> MRVDELRVDERIKSTLKERGIESFYPPQAEALKSGILEGKNALISIPTASGKTLIAEIAMVHRILTQGGKAVYIVPLKALAEEKFQEFQDWEKIGLRVAMATGDYDSKDEWLGKYDIIIATAEKFDSLLRHGSSWIKDVKILVADEIHLIGSRDRGATLEVILAHMLGKAQIIGLSATIGNPEELAEWLNAELIVSDWRPVKLRRGVFYQGFVTWEDGSIDRFSSWEELVYDAIRKKKGALIFVNMRRKAERVALELSKKVKSLLTKPEIRALNELADSLEENPTNEKLAKAIRGGVAFHHAGLGRDERVLVEENFRKGIIKAVVATPTLSAGINTPAFRVIIRDIWRYSDFGMERIPIIEVHQMLGRAGRPKYDEVGEGIIVSTSDDPREVMNHYIFGKPEKLFSQLSNESNLRSQVLALIATFGYSTVEEILKFISNTFYAYQRKDTYSLEEKIRNILYFLLENEFIEISLEDKIRPLSLGIRTAKLYIDPYTAKMFKDKMEEVVKDPNPIGIFHLISLTPDITPFNYSKREFERLEEEYYEFKDRLYFDDPYISGYDPYLERKFFRAFKTALVLLAWINEVPEGEIVEKYSVEPGDIYRIVETAEWLVYSLKEIAKVLGAYEIVDYLETLRVRVKYGIREELIPLMQLPLVGRRRARALYNSGFRSIEDISQARPEELLKIEGIGVKTVEAIFKFLGKNVKISEKPRKSTLDYFLKS

Pyrococcus furiosus Hjm (PfuHjm) is a structure-specific DNA helicase that was originally identified by in vitro screening for Holliday junction migration activity. It belongs to helicase superfamily 2, and shares homology with the human DNA polymerase Θ (PolΘ), HEL308, and Drosophila Mus308 proteins, which are involved in DNA repair. Previous biochemical and genetic analyses revealed that PfuHjm preferentially binds to fork-related Y-structured DNAs and unwinds their double-stranded regions, suggesting that this helicase is a functional counterpart of the bacterial RecQ helicase, which is essential for genome maintenance. PfuHjm folds into five domains (domains 1 to 5) with dimensions of approximately 70 × 50 × 30 Å.

We obtained the two different PfuHjm crystals (Forms 1 and 2) in the nucleotide free-state, and determined their structures at 2.4 Å (Form 1) and 2.0 Å (Form 2) resolutions, respectively. In the Form 1 crystal, the C-terminal 60 residues, about two thirds of the C-terminal domain, are missing in the final model, presumably because of structural disorder. The structures of the two apo-forms are quite similar, with a root-mean square deviation (rmsd) of 1.05 Å for the corresponding 651 Cα atoms. The Form1 crystals were obtained using ammonium sulfate as a precipitant, and it was found that five sulfate ions were bound to the protein. Notably, all of the sulfate ions lie on possible DNA binding surfaces. Collectively, these results indicate that the sulfate/phosphate ions mimic DNA backbone phosphates. For instance, a sulfate ion is strongly bound to Arg306 and Arg309 in domain 2 of PfuHjm. Two point mutations (R306A or R309A) in PfuHjm significantly decreased the DNA binding ability (Fujikane and Ishino, unpublished data). However, the C-terminal segment was invisible in both the Form 1 and Form 2 crystals, suggesting that this segment is highly mobile.> GLEKDFLPLYFGWFLTKKSSETLR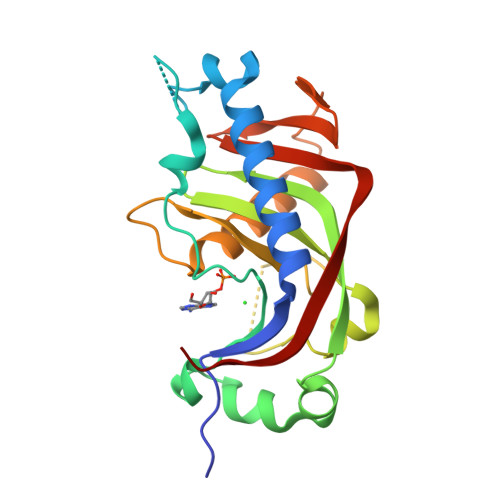KAGQVFLEELGNHKAFKKELRHFISGDEPKEKLELVSYFGKRGPGVLHCTTKFCDYGKAAGAEEYAQQEVVKRSYGKAFKLSISALFVTPKTAGAQVVLTDQELQLWPSDLDKPSASEGLPPGSRAHVTLGCAADVQPVQTGLDLLDILQQVKGGSQGEAVGELPRGKLYSLGKGRWMLSLTKKMEVKAIFTGYYG> MKKNILNLALVGALSTSFLMAKPAHNANNATHNTKKTTDSSAGVLATVDGRPITKSDFDMIKQRNPNFDFDKLKEKEKETLIDQAIRTALVENEAKTEKLDSTPEFKAMMEAVKKQALVEFWAKKQAEEVKKVQIPEKEMQDFYNANKDQLFVKQEAHARHILVKTEDEAKRIISEIDKQPKAKKEAKFIELANRDT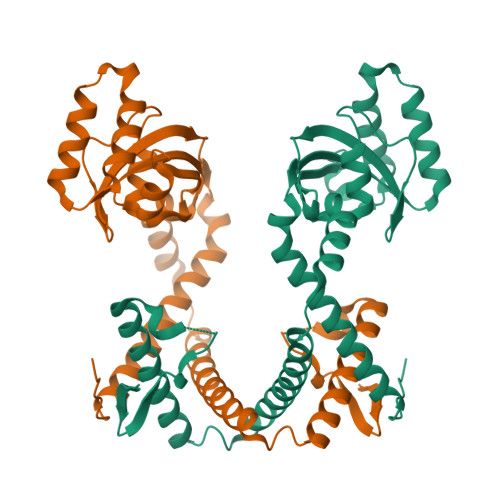IDPNSKNAQNGGDLGKFQKNQMAPDFSKAAFALTPGDYTKTPVKTEFGYHIIYLISKDSPVTYTYEQAKPTIKGMLQEKLFQERMNQRIEELRKHAKIVINK> SERTELLKPRTLADLIRILHELFAGDEVNVEEVQAVLEAYESNPAEWALYAKFDQYRYTRNL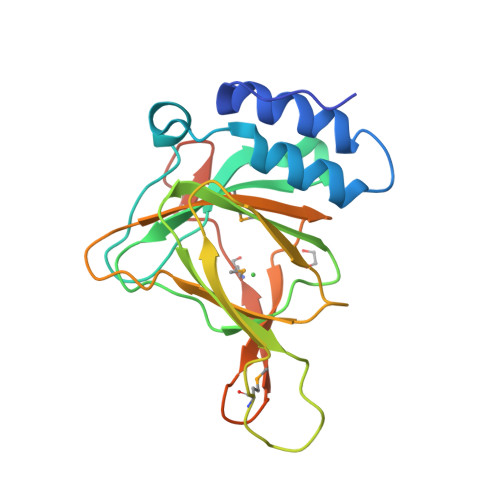VDQGNGKFNLMILCWGEGHGSSIHDHTDSHCFLKLLQGNLKETLFDWPDKKSNEMIKKSERTLRENQCAYINDSIGLHRVENVSHTEPAVSLHLYSPPFDTCHAFDQRTGHKNKVTMTFHSKFGIRTPFTTSGSLENN> MFEQRVNSDVLTVSTVN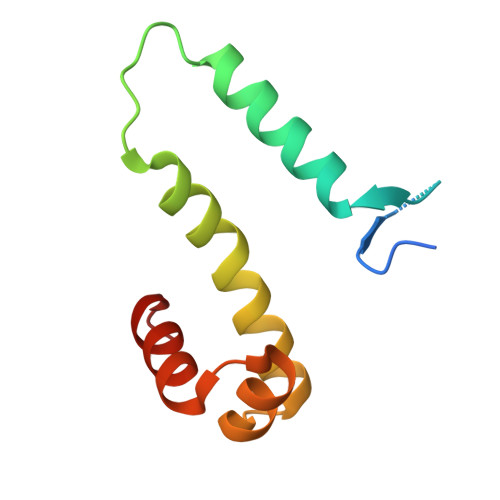SQDQVTQKPLRDSVKQALKNYFAQLNGQDVNDLYELVLAEVEQPLLDMVMQYTRGNQTRAALMMGINRGTLRKKLKKYGMN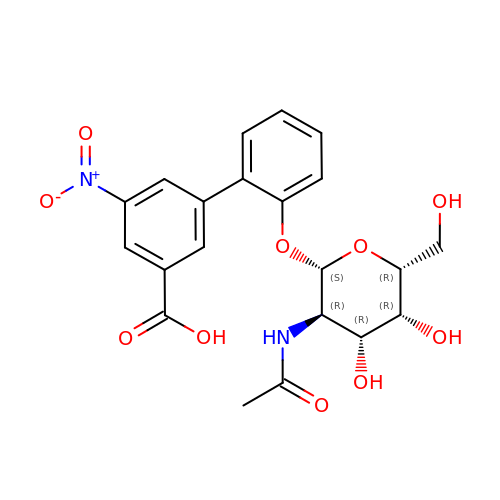2'-{[2-(acetylamino)-2-deoxy-beta-D-galactopyranosyl]oxy}-5-nitro[1,1'-biphenyl]-3-carboxylic acid | C21 H22 N2 O10 | MUERTXQUUVQXJH-GQUPQBGVSA-N> VQIHDITGKDCQDIANKGAKQSGLYFIKPLKANQQFLVYCEIDGSGNGWTVFQKRLDGSVDFKKNWIQYKEGFGHLSPTGTTEFWLGNEKIHLISTQSAIPYALRVELEDWNGRTSTADYAMFKVGPEADKYRLTYAYFAGGDAGDAFDGFDFGDDPSDKFFTSHNGMQFSTWDNDNDKFEGNCAEQDGSGWWMNKCHAGHLNGVYYQGGTYSKASTPNGYDNGIIWATWKTRWYSMKKTTMKIIPF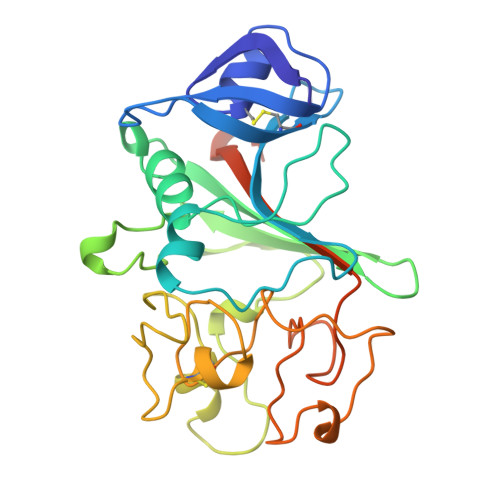NRLTIGEGQQHHLGGAKQAGDV>[4x]TDPALRAITHISPLGSMDMLSQLEVDMLKRTASSDLYQLFRNCSLAVLNSGSLTDNSKELLSRFENFDINVLRRERGVKLELINPPEE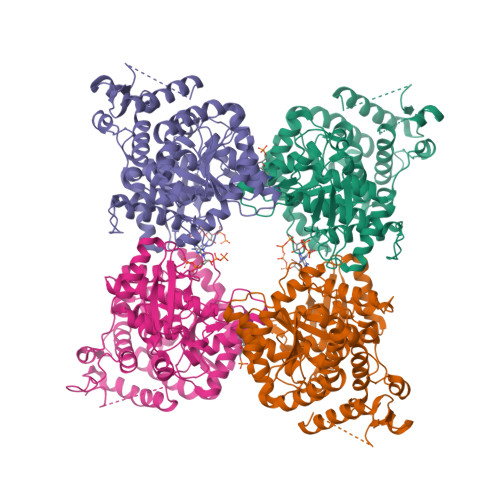AFVDGRIIRALQANLFAVLRDILFVYGQIHNTVRFPNLNLDNSVHITNLVFSILRNARALHVGEAPNMVVCWGGHSINENEYLYARRVGNQLGLRELNICTGCGPGAMEAPMKGAAVGHAQQRYKDSRFIGMTEPSIIAAEPPNPLVNELIIMPDIEKRLEAFVRIAHGIIIFPGGVGTAEELLYLLGILMNPANKDQVLPLILTGPKESADYFRVLDEFVVHTLGENARRHYRIIIDDAAEVARQMKKSMPLVKENRRDTGDAYSFNWSMRIAPDLQMPFEPSHENMANLKLYPDQPVEVLAADLRRAFSGIVAGNVKEVGIRAIEEFGPYKINGDKEIMRRMDDLLQGFVAQHRMKLPGSAYIPCYEICT> MVDQH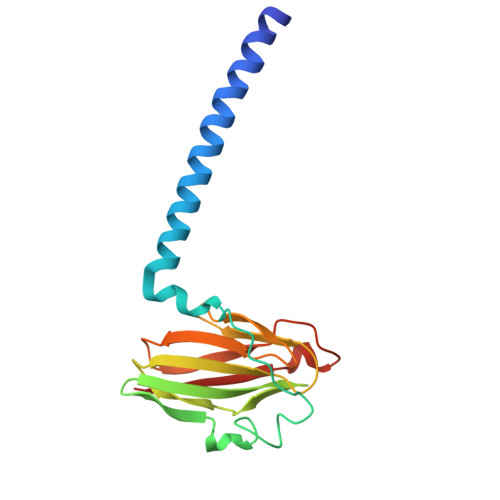KAHKAILAYEKGWLAFSLAMLFVFIALIAYTLATHTAGVIPAGKLERVDPTTVRQEGPWADPAQAVVQTGPNQYTVYVLAFAFGYQPNPIEVPQGAEIVFKITSPDVIHGFHVEGTNINVEVLPGEVSTVRYTFKRPGEYRIICNQYCGLGHQNMFGTIVVKE>MKSVITTVVSAADAAGR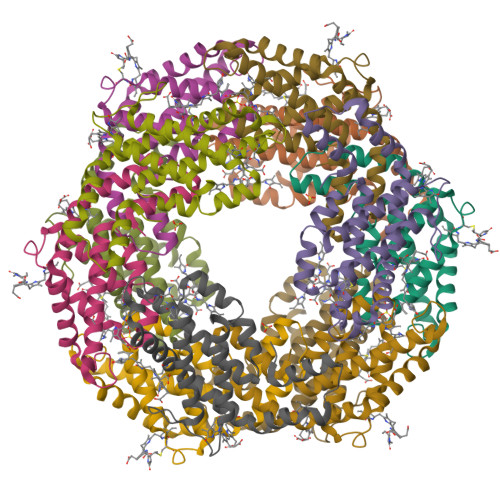FPSNSDLESIQGNIQRSAARLEAAEKLAGNHEAVVKEAGDACFAKYAYLKNPGEAGENQEKINKCYRDVDHYMRLVNYCLVVGGTGPLDEWGIAGAREVYRTLNLPTSAYVASIAYTRDRLCVPRDMSAQAGVEFSAYLDYLINALS[2x];>[2x]MLDAFSRVVVNSDAKAAYVGGSDLQALKSFIADGNKRLDAVNSIVSNASCMVSDAVSGMICENPGLISPGGNCYTNRRMAACLRDGEIILRYVSYALLAGDASVLEDRCLNGLKETYIALGVPTNSSIRAVSIMKAQAVAFITNTATERKMSFAAGDCTSLASEVASYFDRVGAAIS> M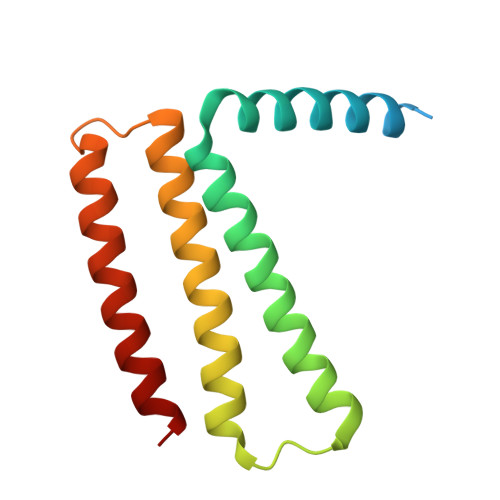AKAPKANTPKVTSTSSAVLTDFQETFKTSKRAYFAQIEKYPKLKLIDTFCFFLVLLGVIQCTFIILIRDNFPFNAFLAGFIICVGQFVLLMSLRLQLCNSFPGISKNRAFAEFIVASLILHFVCLHFIN>[2x]MNNMNVIIADDHPIVLFGIRKSLEQIEWVNVVGEFEDSTALINNL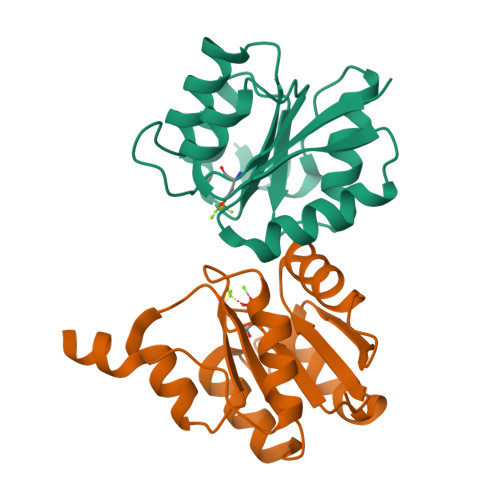PKLDAHVLITDLSMPGDKYGDGITLIKYIKRHFPSLSIIVLTMNNNPAILSAVLDLDIEGIVLKQGAPTDLPKALAALQKGKKFTPESVSRLLEKISA> MKEEVKGIPVRVALRCRPLVSKEIKEGCQTCLSFVPGEPQVVVGNDKSFTYDFVFDPSTEQEEVFNTAVAPLIKGVFKGYNATVLAYGQTGSGKTYSMGGAYTAEQEHDSAIGVIPRVIQLLFKEINKKSDFEFTLKVSYLEIYNEEILDLLCSSREKATQINIREDPKEGIKIVGLTEKTVLVAS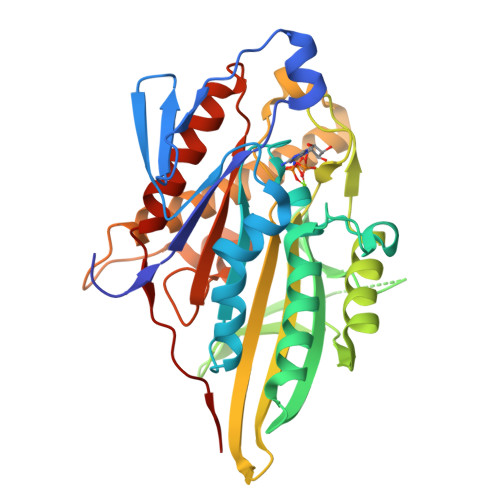DTVSCLEQGNNSRTVASTAMNSQSSRSHAIFTISIEQRKKNDKNSSFRSKLHLVDLAGSERQKKTKAEGDRLREGININRGLLCLGNVISALGDDKKGNFVPYRDSKLTRLLQDSLGGNSHTLMIACVSPADSNLEETLNTLRYADRARKIKNKPIINHHHHHH> MNNNKAEADTSSSMADPETRPTYTTHHLAIPSGVTQDEFDELKQSVVEFHTYQLSQAQCSSLLAQRIRAPNDVVWSIVRRFDQPQTYKHFIKSCSVSDNFTMAVGSTRDVNVISGLPAATSTERLDILDDDRQVTGFSIIGGEHRLRNYRSVTSVHGFNRDGAICTVVLESYVVDVPEGNTEEDTRLFADTVVKLNLQKLVSVAESQVI;> RSVYELDCIPLWGVVSIQGNRSEMEDAFAVSPHFLKLPIKMLMGDHEGMSPSATHLTGHFFGVYDGHGGHKVADYCRDRLHFALAEEIERIKDELCKRNTGEGRQVQWDKVFTSCFLTVDGEIEGKIGRAVVGSSDKVLEAVASETVGSTAVVALVCSSHIVVSNCGDSRAVLFRGKEAMPL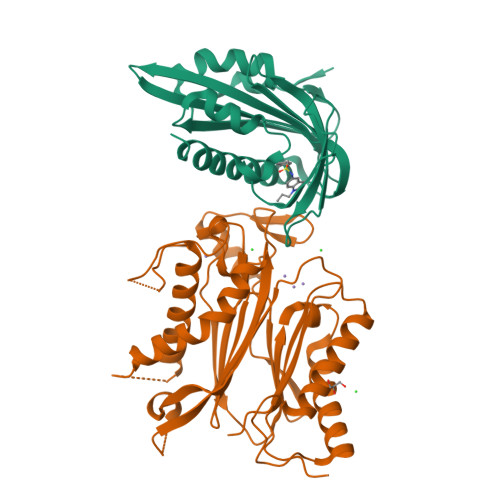SVDHKPDREDEYARIENAGGKVIQWQGARVFGVLAMSRSIGDRYLKPYVIPEPEVTFMPRSREDECLILASDGLWDVMNNQEVCEIARRRILMWHKKNGAPPLAERGKGIDPACQAAADYLSMLALQKGSKDNISIIVIDLKAQRKFKTRT3-thiaglutaryl-CoA | 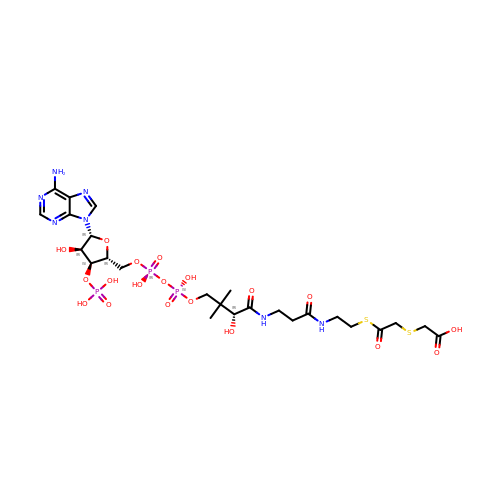C25 H40 N7 O19 P3 S2 | GKSSRSUPHZUOQO-ITIYDSSPSA-N>[2x]GSHMAGNDSNLIWLDLEMTGLEPV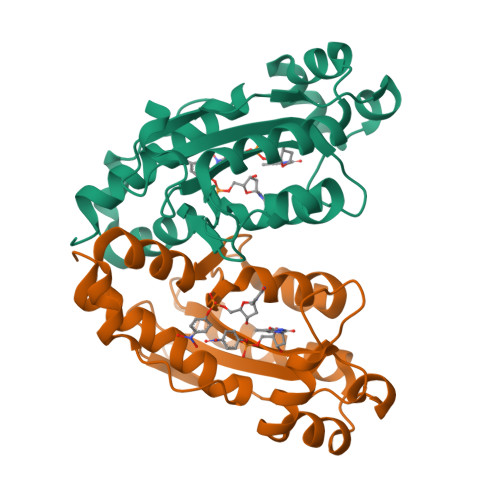EDVILEIAIIITDSELNILAQGPIFAISQTDDVLDNMNPWCIEHHGKSGLTQRCRDSEVSLAHATKESLAFVQEWVPQGKSPMCGNSIGQDRRFINKYMPDFEDHFHYRNLDVSTIKELAKRWKPEVLESVVKTGAHLALDAIKESIAELKVYRELFFKL> MAHHHHHHVGTGDWRTATSMHEFSVPDIDGNMVNLDQYRGKTVIVTNVASQCGKTEVNYTQLVELHRKHRAEGLEILAFPCNQFGKQEPGSNEEIKAFCAQYNVTFHMFSKIDVNGADAHPLWKWLKVQPNG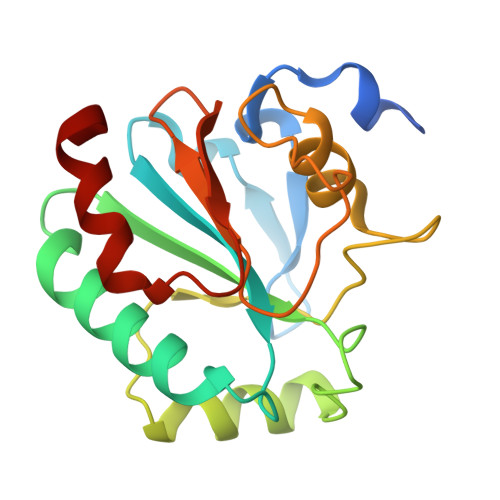QGVGGNAIKWNFTKFLIDKNGKVVKRYGPMTEPRDIEADLPKYF>SNAMKIAVINGGTRSGGNTDVLAEKAVQGFDAEHIYLQKYPIQPIEDLRHAQGGFRPVQDDYDSIIERILQCHILIFATPIYWFGMSGTLKLFIDRWSQTLRDPRFPDFKQQMSVKQAYVIAVGGDNPKIKGLPLIQQF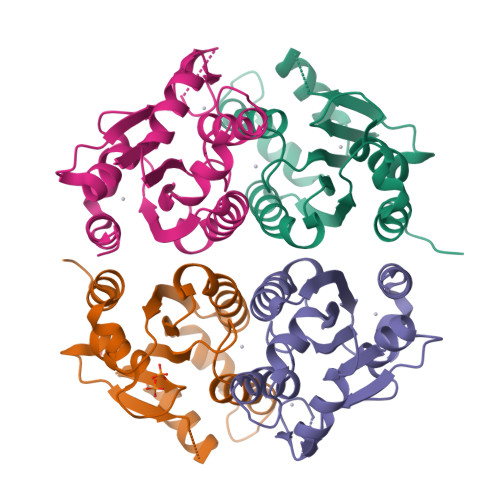EHIFHFMGMSFKGYVLGEGNRPGDILRDHQALSAASRLLKRSDAI[4x]4-(2-METHOXYPHENYL)-2-OXOBUT-3-ENOIC ACID | C11 H10 O4 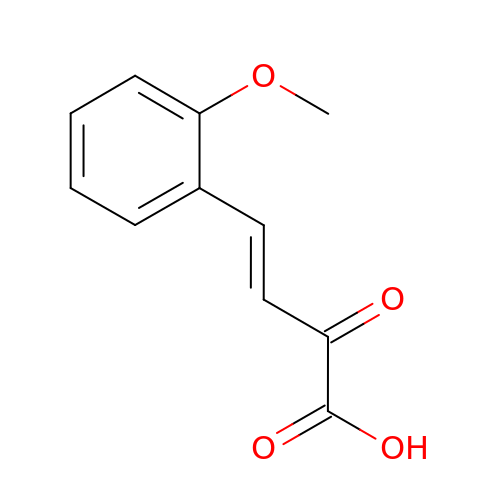| QGTBUESLYPYXRT-SREVYHEPSA-N N-Acyl homoserine lactonases (AHL-lactonases) have important functions in decreasing pathogenicity by degrading AHLs. Unlike most AHL-lactonases, AidH is proposed to be a member of the α/β-hydrolase fold family. AidH contains a substrate-binding tunnel between the core domain and the cap domain. Taken together, the present results reveal the catalytic mechanism of the metal-independent AHL-lactonase, which is a typical acid–base covalent catalysis.

Surprisingly, the mutant AidHE219G is not completely inactive and the activity of AidHY160G is significantly decreased. The biochemical data demonstrate that the Glu219→Gly mutation weakens the His-dependent solvent-assisted deprotonation and thus decreases the activity of AidH. Throughout the reaction, the carboxyl group of Glu219 forms a hydrogen bond to His248, giving it the correct conformation and the proper tautomeric equilibrium after it accepts the proton from Ser102.

>MTINYHELETSHGRIAVRESEGEGAPLLMIHGNSSSGAIFAPQLEGEIGKKWRVIAPDLPGHGKSTDAIDPDRSYSMEGYADAMTEVMQQLGIADAVVFGWSLGGHIGIEMIARYPEMRGLMITGTPPVAREEVGQGFKSGPDMALAGQEIFSERDVESYARSTCGEPFEASLLDIVARTDGRARRIMFEKFGSGTGGNQRDIVAEAQLPIAVVNGRDGPFVELDFVSKVKFGNLWEGKTHVIDNAGHAPFREAPAEFDAYLARFIRDCTQLEHHHHHH[2x]>MSNKCDVVVVGGGISGMAAAKLLHDSGLNVVVLEARDRVGGRTYTLRNQKVKYVDLGGSYVGPTQNRILRLAKELGLETYKVNEVERLIHHVKGKSYPFRGPF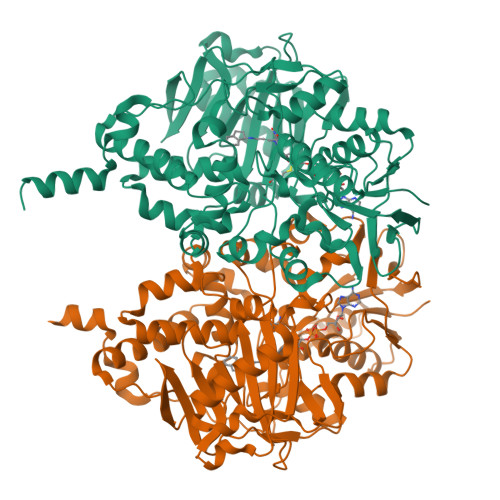PPVWNPITYLDHNNFWRTMDDMGREIPSDAPWKAPLAEEWDNMTMKELLDKLCWTESAKQLATLFVNLCVTAETHEVSALWFLWYVKQCGGTTRIISTTNGGQERKFVGGSGQVSERIMDLLGDRVKLERPVIYIDQTRENVLVETLNHEMYEAKYVISAIPPTLGMKIHFNPPLPMMRNQMITRVPLGSVIKCIVYYKEPFWRKKDYCGTMIIDGEEAPVAYTLDDTKPEGNYAAIMGFILAHKARKLARLTKEERLKKLCELYAKVLGSLEALEPVHYEEKNWCEEQYSGGCYTTYFPPGILTQYGRVLRQPVDRIYFAGTETATHWSGFMEGAVEAGERAAREILHAMGKIPEDEIWQSEPESVDVPAQPITTTFLERHLPSVPGLLRLIGLTTIFSATALGFLAHKRGLLVRV[2x]> MDEKLLKTIAESKYLVALTGAGVSAESGIPTFRGKDGLWNRYRPEELAN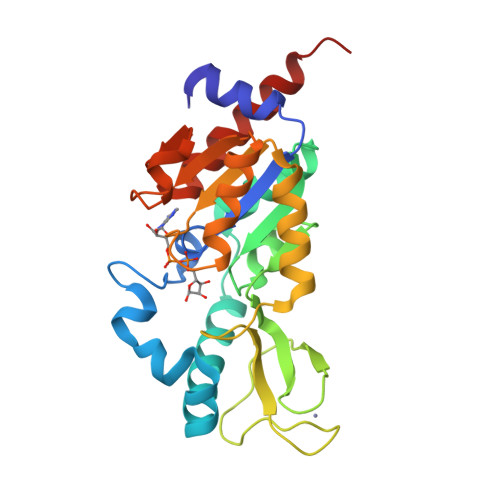PQAFAKDPEKVWKWYAWRMEKVFNAQPNKAHQAFAELERLGVLKCLITQNVDDLHERAGSRNVIHLHGSLRVVRCTSCNNSFEVESAPKIPPLPKCDKCGSLLRPGVVWFGEMLPPDVLDRAMREVERADVIIVAGTSAVVQPAASLPLIVKQRGGAIIEINPDETPLTPIADYSLRGKAGEVMDELVRHVRKALSLKLN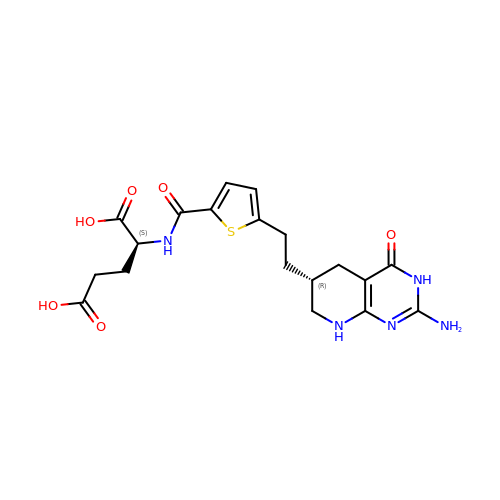N-[(5-{2-[(6R)-2-AMINO-4-OXO-3,4,5,6,7,8-HEXAHYDROPYRIDO[2,3-D]PYRIMIDIN-6-YL]ETHYL}-2-THIENYL)CARBONYL]-L-GLUTAMIC ACID | C19 H23 N5 O6 S | GQCXGHHHNACOGE-SKDRFNHKSA-N> GPG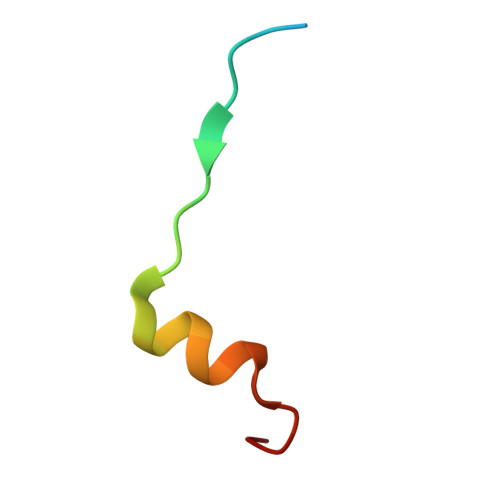SQPTRRQIRLSSPERQRLSSLNLT>[2x]MTSSSTPRHRGIFPVVPTTFADTGDLDLASQKRAV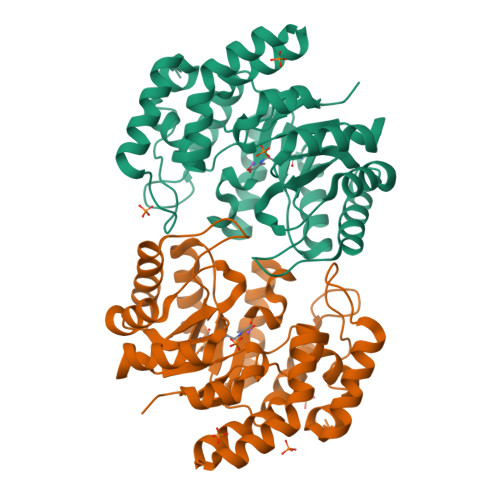DFMIDAGSDGLCILANFSEQFAITDDERDVLTRTILEHVAGRVPVIVTTSHYSTQVCAARSLRAQQLGAAMVMAMPPYHGATFRVPEAQIFEFYARVSDAIAIPIMVQDAPASGTALSAPFLARMAREIEQVAYFKIETPGAANKLRELIRLGGDAIEGPWDGEEAITLLADLHAGATGAMTGGGFPDGIRPILEAWREGRHDDAYARYQAWLPLINHENRQSGILTAKALMREGGVIASERPRHPMPELHPDTRAELLAIARRLDPLVLRWAH> MAILAFQKPENVLMMETSDSIAKFEFKPLEPGYGITIGNALRRILLSSLEGFAITAIKIEGVEHEFATIPGVLEDVTNIILNLKQVRFKQIVPNADVEKATIVISNSEVFRAGDLNAQLSNFEVLNSNLVICHLDKSATLTMEFSINKGRGYVSAEENRAEHNELSTIAIDS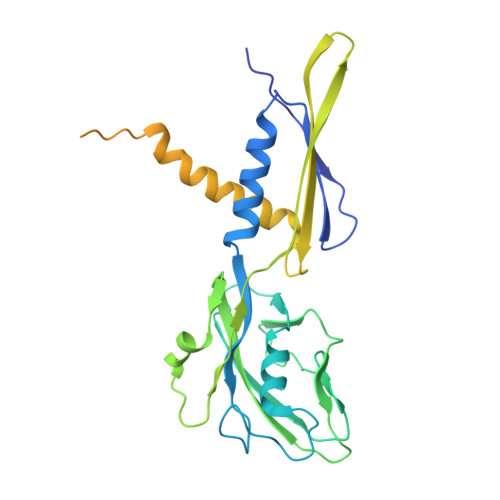IYTPIRNVKYAVENFRVEQKTDYEKLLMEVTTDGSIRPVDALREAAQILISHFSLFAENKIAIEYVDIVDTDEFDEDSLHMRQLLKSKLSGLDLSVRALNCLNAAGVDTLGDLVSLSRSDLMKIRNFGKKSLTELDELLATLNLSFGMDISKYKLDKD>[2x]LSGDAVQKMLGHCTFEPAEPKAAKNTYTAERFIWLTKLNNLRILEQGSERPLTDTERATLMDEPYRKSKLTYAQARKLLGLEDTAFFKGLRYGK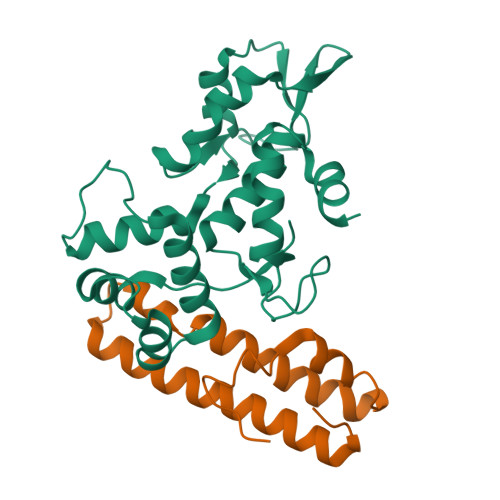DNAEASTLMEMKAYHAISRALEKEGLKDKKSPLNLSPELQDEIGTAFSLFKTDEDITGRLKDRIQPEILEALLKHISFDKFVQISLKALRRIVPLMEQGKRYDEACAEIYGDHY;>MKITSSNFATIATSENFAKLSVLPKNHREPIKGLFKSAVEQFSSARDFFKNENYSKELAEKFNKEAVNEAVEKLQKAIDLAEKQGIQF[2x]>GHMAVPDDDDDDDNSNDESEYESSQMDSEKNKGSIKNSKNVVIYADGVYDMLHLGHMKQLEQAKKLFENTTLIVGVTSDNETKLFKGQVVQTLEERTETLKHIRWVDEIISPCPWVVTPEFLEKYKIDYVAHDDIPYANNQKEDIYAWLKRAGKFKATQRTEGVSTTDLIVRILKNYEDY[6x]

The de novo Kennedy pathway is the main route for the PC synthesis in P. falciparum and has been identified as a pharmacological target for the treatment of malaria. In contrast, the gene of PfCCT underwent a domain duplication event and thus encodes two catalytic and two membrane binding domains connected by a disordered interdomain segment. Here, we present the crystal structures of the catalytic domain of the P. falciparum enzyme (PfCCT) in the free form, as well as in complex with its substrate ChoP or fragments (CMP and choline) and with the product CDPCho, thereby visualizing the free and the ChoP-complexed states of CCT for the first time. The enzyme forms a globular dimer with an α/β Rossmann fold that is well conserved in CCTs and other members of the cytidylyltransferase enzyme family.

The major change concerned loop L5 (residues 712–738) that is only visible in the presence of CDPCho. In this case, ordered conformation of the loop is assisted by the interaction of Y714 with the ligand which is apparently not strong enough with ChoP or choline to render loop L5 ordered. Intriguingly, loop L5 hardly establishes contacts to other structural elements, thus its anchoring to the active site is presumably fostered by the cation-π and polar interactions of Y714 with CDPCho. Closure of the choline subsite in the CDPCho-bound state is also accompanied by the further inward movement of I740 and Y741. Meanwhile, K663 moves to coordinate the Pα group in addition to the Pβ group of CDPCho that originated from ChoP, allowing the phenolic OH of Y714 to coordinate Pβ moiety. The nucleotide ligands CMP and CDPCho are anchored in the active site by several polar contacts, hydrogen bonds and a cation-π interaction of R755 with the cytosine ring. The coordination of the nucleophile phosphate moiety in ChoP- and CDPCho-liganded structures is ensured by V625, K663 and H709 residues. CDPCho is found in the same zig-zag position in both PfCCT and RnCCT co-structures with only the two methylene groups of this ligand adopting different conformations. A notable structural difference involves Q636 sidechain that enables a direct interaction with the ribose 3′OH moiety in PfCCT, whereas a similar contact in RnCCT is established by an ordered water molecule next to A95.Orai was identified as the protein that forms the channel’s pore and STIM was identified as its regulator. The channel is activated by the depletion of Ca2+ from the endoplasmic reticulum (ER), and as such it was characterized as the calcium release-activated calcium (CRAC) channel responsible for store-operated calcium entry (SOCE) before the molecular components were known. The channel is formed from an assembly of six Orai subunits that surround a single ion pore, which is perpendicular to the plasma membrane in a cellular setting. Each Orai subunit contains four transmembrane helices (M1-M4) and a cytosolic M4-ext helix.

In this study, we introduced the corresponding amino acid substitution into Drosophila Orai (H206A), confirmed that it generates a constitutively active channel, and determined its X-ray structure. Thus, as has been shown for the corresponding H134A mutation of human Orai1, H206A Oraicryst forms an open channel that recapitulates properties of STIM-activated Orai. Extensive optimization of crystallization conditions improved the quality of H206A Oraicryst crystals from an initial diffraction limit of 20 Å resolution to 6.7 Å resolution. In this case, the asymmetric unit contains 24 Orai subunits, which are arranged as four complete channels. The X-ray structure of H206A Oraicryst reveals a new conformation of the channel with a dilated pore that presumably represents an open conformation. In comparison to the closed pore, the pore is dramatically dilated on its cytosolic end, expanding by ~10 Å at Lys159. The electron density indicates that the principal conformational change in the pore results from an outward rigid body rotation of the M1-M4a portion of each subunit away from the central axis and a slight additional outward bend of M1 on its intracellular half. Residue 206 is located on the M2 helix and does not line the pore. In the H206A Oraicryst structure, M4b and M4-ext are repositioned by straightenings of both bends such that the regions corresponding to M4a, M4b and M4-ext of each subunit form a continuous α-helix that traverses the membrane and extends ~45 Å into the cytosolic space. Anomalous difference electron density for iron is not observed in the structure of H206A Oraicryst, indicating that the iron complex is not present in the open pore, which is in accord with the dramatic widening of the basic region.

>MSQSGEDLHSPTYLSWRKLQLSRAKLKASSKTSALLSGFAMVAMVEVQLDHDTNVPPGMLIAFAICTTLLVAVAMLALMISTCILPNIETVSNLHSISLVHESPHERLHWYIETAWAFSTLLGLILFLLEIAILCWVKFYDLSPPAAWSATVVLIPVMIIFMAFAIHFYRSLVSHKYEVTVSGIRELEMLKEQMEQDHLEHHNNIRNNGEGEEF[24x]> MLVRLLRVILLASMVFCADILQLSYSDDAKDAIPLGTFEIDSTSDGNVTVTTVNIQDVEVSGEYCLNAQIEGKLDMPCFSYMKLRTPLKYDLIVDVDEDNEVKQVSLSYDETNDAITATVRYPEAGPTAPVTKLKKKTKTYADKKASKNKDGSTAQFEEDEEVKEVSWFQKNWKMLLLGLLIYNFVAGSAKKQQQGGAGADQKTE;> MKITCTDLVYVFILLFLNTSCVQAVFSDDAFITDWQLANLGPWEKVIPDSRDRNRVLILSNPTETSCLVSSFNVSSGQILFRNVLPFTIDEIQLDSNDHNAMVCVNSSSNHWQKYDLHDWFLLEEGVDNAPSTTILPQSSYLNDQVSIKNNELHILDEQSKLAEWKLELPQGFNKVEYFHREDPLALVLNVNDTQYMGFSANGTELIPVWQRDEWLTNVVDYAVLDVFDSRDVELNKDMKAELDSNSLWNAYWLRLTTNWNRLINLLKENQFSPGRVFTKLLALDAKDTTVSDLKFGFAKILIVLTHDGFIGGLDMVNKGQLIWKLDLEIDQGVKMFWTDKNHDELVVFSHDGHYLTIEVTKDQPIIKSRSPLSERKTVDSVIRLNEHDHQYLIKFEDKDHLLFKLNPGKNTDVPIVANNHSSSHIFVTEHDTNGIYGYIIENDTVKQTWKKAVNSKEKMVAYSKRETTNLNTLGITLGDKSVLYKYLYPNLAAYLIANEEHHTITFNLIDTITGEILITQEHKDSPDFRFPMDIVFGEYWVVYSYFSSEPVPEQKLVVVELYESLTPDERLSNSSDNFSYDPLTGHINKPQFQTKQFIFPEIIKTMSISKTTDDITTKAIVMELENGQITYIPKLLLNARGKPAEEMAKDKKKEFMATPYTPVIPINDNFIITHFRNLLPGS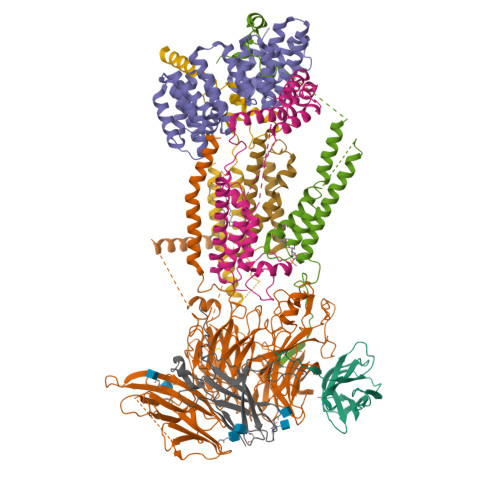DSQLISIPTNLESTSIICDLGLDVFCTRITPSGQFDLMSPTFEKGKLLITIFVLLVITYFIRPSVSNKKLKSQWLIK;> MLKDLVREKLLTIMNTKAYTQFNPEQLLQLENEMKIYMKSGDSALTEGNYFFLMEMLFYVLVYRNQDVDAQVVYNTLRDRLGENSYKMVIMKATLLQINGNDKGAIEYLENLLNDDLEYETDFVTYVSIAKKLIAIKTTSKNLSQESVLKEVVALTDKFPLDAELWWYASEIYFEMGQFEKACYCLEQVLCITPFNYACFGRLSETLYYEALRSKKQTKTELLEKALKNALRSVELSELYLKGWALVNIISRELGRNKQNDLIKLSASKLKEISAKSNNKDKITAELILNKI;> MLLDDQLKYWVLLPISIVMVLTGVLKQYIMTLITGSSANEAQPRVKLTEWQYLQWAQLLIGNGGNLSSDAFAAKKEFLVKDLTEERHLAKAKQQDGSQAGEVPNPFNDPSMSNAMMNMAKGNMASFIPQTIIMWWVNHFFAGFILMQLPFPLTAKFKEMLQTGIICQDLDVRWVSSISWYFISVLGLNPVYNLIGLNDQDMGIQAGIGGPQGPQGPPQSQVDKAMHAMANDLTIIQHETCLDNVEQRVLKQYM;> MSEQEPYEWAKHLLDTKYIEKYNIQNSNTLPSPPGFEGNSSKGNVTRKQQDATSQTTSLAQKNQITVLQVQKAWQIALQPAKSIPMNIFMSYMSGTSLQIIPIMTALMLLSGPIKAIFSTRSAFKPVLGNKATQSQVQTAMFMYIVFQGVLMYIGYRKLNSMGLIPNAKGDWLPWERIAHYNNGLQWFSD;> MSFVSKLLYTVSALVLFHSGFSSYEFHHLLKLNSLNNAQGAISKLPKDIMYETYAGLILFVLAVFTSFEKLQYLPIESNDGKIISQGNYLKEIALNKATNVDNLIGSNPNGEIIFTPSFVDVHMKRKICREWASNTVKKEK;> MSSNEEVFTQINATANVVDNKKRLLFVQDSSALVLGLVAGFLQIESVHGFIWFLILYNLINVIYIVWICQLQPGKFYQSPLQDIFFESFFREITGFVMAWTFGYALIG;> MFSQIVLLLSAFIYVASATARRGTIKGRLDLAASNITGFVSTRTSFKLYQIGNFSTEYPYTSTTMFQDDEGNFEFANLPLNDGVNETTYYVMYPASMDFNLKPNRILIEFKNLENGTLQLNAFKNFFGREYFPSKDITYPEKLQSMKVHPYITVELLHKAPIRSYLQARNVSIFSTGIVGNILNSRWKLAGVITLIALVVFPIIVEKLDPETARAIREEAKRKQREKYAAVASK Sulfatinib is a multi-target drug that selectively targets FGFR, collection stimulating factor 1 receptor (CSF-1R), and vascular endothelial growth factor receptor (VEGFR). To achieve this, we determined the crystal structures of sulfatinib in complex with FGFR1 and CSF-1R using X-ray crystallography. Sulfatinib exhibits dramatic conformational changes upon FGFR1 and CSF-1R except for the hinge-interacting pattern. Notably, the flexibility provided by the oxy linker of sulfatinib emerges as a critical factor for the FGFR and CSF-1R targeting, allowing sulfatinib to adapt and adopt multiple binding conformations in response to different kinase bindings.

Specifically, CSF-1R adopts a DFG-out activation loop upon sulfatinib binding. Sulfatinib maps in the ATP-binding pocket of CSF-1R with the pyrimidine nitrogen and the adjacent phenylamine NH making a bidentate hydrogen bond with the hinge residue Cys666 and the N-(2-dimethylamino-ethyl)-ethanesulfonamide moiety extending toward the solvent-exposed area. Unexpectedly, the indole group of sulfatinib does not occupy the hydrophobic pocket but rotates out in response to the DFG-out flip. These results demonstrate that sulfatinib inhibits CSF-1R by locking the protein in an inactive state, classified as a type II inhibitor. The indole group of sulfatinib in CSF-1R is flipped out of the hydrophobic pocket via an oxy linker. In contrast, the solubilizing group is rotated by 180° in proximity to the hinge region of CSF-1R, compared with that of FGFR1. We supposed that sulfatinib may bind to CSF-1R as the mode with FGFR1, but the indole group of sulfatinib may clash with Lys616 and Phe797 of CSF-1R, which means it may have a higher-energy barrier to attain the FGFR1-sulfatinib binding mode. As to CSF-1R, the R-spine is broken and Phe797 is displaced by Trp550 from the juxtamembrane domain (JMD), thereby forcing the DFG-out flip and forming an inhibitory R-spine. The kinase activity inhibition assay results showed that sulfatinib preserved a remarkable inhibitory effect on CSF-1RT663I with IC50 value of 4 nM. It seems that there is a large space available to accommodate sulfatinib without steric clash with the isoleucine side chain, supporting the high sustainability of sulfatinib against CSF-1RT663I mutation as determined by biochemical assay.

> MKKGHHHHHHGQKPKYQVRWKIIESYEGNSYTFIDPTQLPYNEKWEFPRNNLQFGKTLGAGAFGKVVEATAFGLGKEDAVLKVAVKMLKSTAHADEKEALMSELKIMSHLGQHENIVNLLGACTHGGPVLVITEYCTYGDLLNFLRRKAEAMLGPSLSPGQDPEGGVDYKNIHLEKLDKEDGRPLELRDLLHFSSQVAQGMAFLASKNCIHRDVAARNVLLTNGHVAKIGDFGLARDIMNDSNYIVKGNARLPVKWMAPESIFDSVYTVQSDVWSYGILLWEIFSLGLNPYPGILVNSKFYKLVKDGYQMAQPAFAPKNIYSIMQACWALEPTHRPTFQQITSFLQEQAQEDRR>MKHLTTMSELSTEEIKDLLQTAQELKSGKTDNQLTGKFAANLFFEPSTRTRFSFEVAEKKLGMNVLNLDGTSTSVQKGETLYDTIRTLESIGVDVCVIRHSEDEYYEELVSQVNIPILNAGDGCGQHPTQSLLDL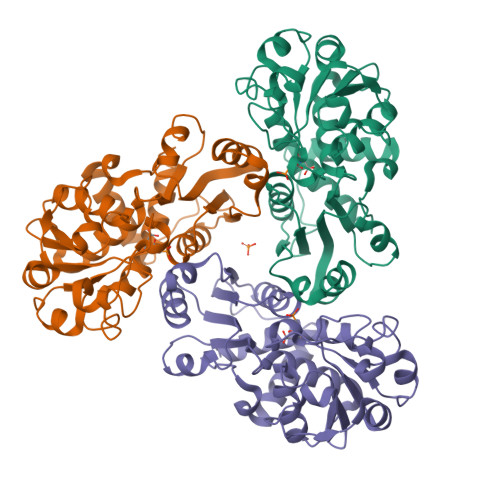MTIYEEFNTFKGLTVSIHGDIKHSRVARSNAEVLTRLGARVLFSGPSEWQDEENTFGTYVSMDEAVESSDVVMLLRIQNERHQSAVSQEGYLNKYGLTVERAERMKRHAIIMHPAPVNRGVEIDDSLVESEKSRIFKQMKNGVFIRMAVIQRALQTNVKRGEAAYVISH[6x]>[22x]MYTNSDFVVIKALEDGVNVIGLTRGADTRFHHSEKLDKGEVLIAQFTEHTSAIKVRGKAYIQTRHGVIESEGKK

Specific damage manifestations were determined within the large trp RNA-binding attenuation protein (TRAP) bound to a single-stranded RNA that forms a belt around the protein. TRAP consists of 11 identical subunits assembled into a ring with 11-fold rotational symmetry. For crystalline complexes such as C.Esp1396I, whether the protein is intrinsically more susceptible to X-ray-induced damage or whether the protein scavenges electrons to protect the DNA remains unclear in the absence of a non-nucleic acid-bound protein control obtained under exactly the same crystallization and data-collection conditions. To monitor the effects of nucleic acid binding on protein damage susceptibility, a crystal containing two protein molecules per asymmetric unit, only one of which was bound to RNA, is reported here. In this structure, the bases of the G1-A2-G3 nucleotides form direct hydrogen bonds to the protein, unlike the U4-U5 nucleotides, which appear to be more flexible.

Here, a methodology has been developed whereby per-atom density changes could be quantified with increasing dose over a wide (1.3–25.0 MGy) range and at higher resolution (1.98 Å) than the previous systematic specific damage study on a protein–DNA complex. To quantify the exact effects of nucleic acid binding to a protein on SRD susceptibility, a high-throughput and automated pipeline was created to systematically calculate the electron-density change for every refined atom within the TRAP–RNA structure as a function of dose. This provides an atom-specific quantification of density–dose dynamics, which was previously lacking within the field. The availability of two TRAP molecules in the asymmetric unit, of which only one contained bound RNA, allowed a controlled investigation into the exact role of RNA binding in protein specific damage susceptibility. By employing the high 11-fold structural symmetry within each TRAP macromolecule, this approach permitted a thorough statistical quantification of the RD effects of RNA binding to TRAP.2-methyl-3-(1~{H}-pyrazol-5-yl)imidazo[1,2-a]pyridine | C11 H10 N4 | 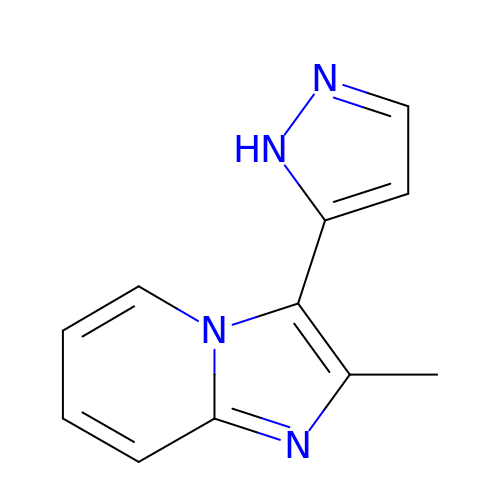HPJHIZQUPBRFBY-UHFFFAOYSA-N>[2x]GAFEDRDPTQFEERHLKFLQQLGKGNFGSVEMCRYDPLQDNTGEVVAVKKLQHSTEEHLRDFEREIEILKSLQHDNIVKYKGVCYSAGRRNLKLIMEYLPYGSLRDYLQAHAERIDHIKLLQYTSQICKGMEYLGTKRYIHRDLATRNILVENENRVKIGDFGLTKVLPQDKEYYKVKEPGESPIFWYAPESLTESKFSVASDVWSFGVVLYELFTYIEKSKS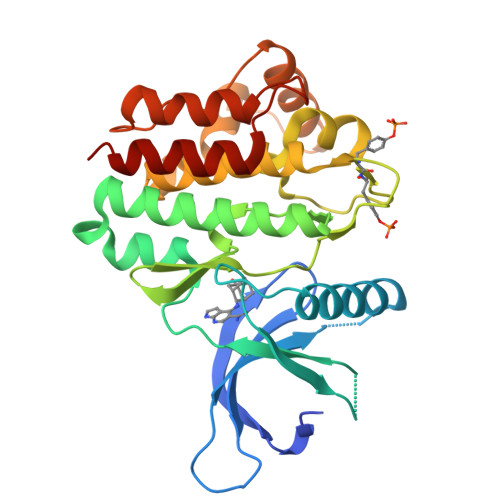PPAEFMRMIGNDKQGQMIVFHLIELLKNNGRLPRPDGCPDEIYMIMTECWNNNVNQRPSFRDLALRVDQIRDNMAG>[9x]MQRLFLLVAVMLLSGCLTAPPKEAARPTLMPRAQSYKDLTHLPAPTGKIFVSVYNIQDETGQFKPYPASNFSTAVPQSATAMLVTALKDSRWFIPLERQGLQNLLNERKIIRAAQENGTVAINNRIPLQSLTAANIMVEGSIIGYESNVKSGGVGARYFGIGADTQYQLDQIAVNLRVVNVSTGEILSSVNTSKTILSYEVQAGVFRFIDYQRLLEGEVGYTSNEPVMLCLMSAIETGVIFLIND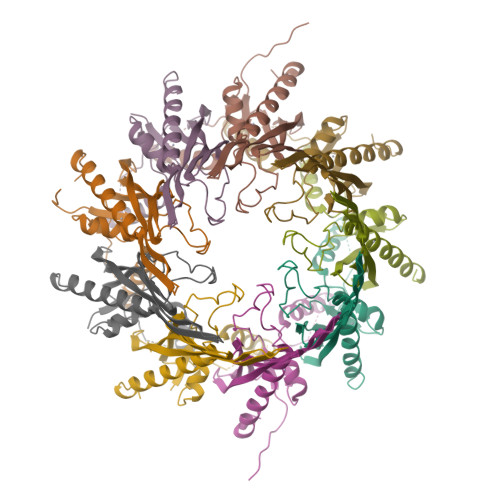GIDRGLWDLQNKAERQNDILVKYRHMSVPPES> LAAMKNFAEQYAKRTDTYFCSDLSVTAVVIEGLARHKEELGSPLCPCRH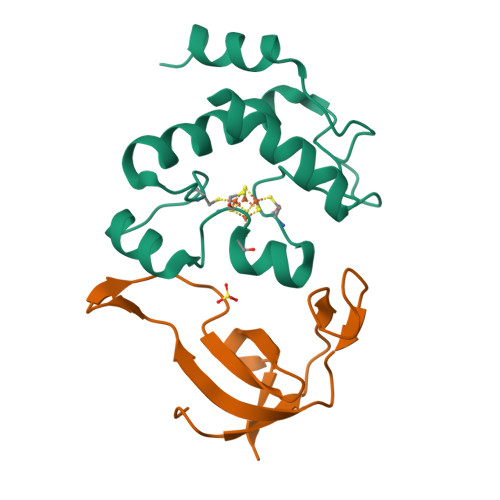YADKEAEVKNTFWNCPCVPMRERKECHCMLFLTPDNDFAGDAQGIPMETLEEKKASMA;> MNVGDRVRVTSSVVVYHHPEHAKTAFDLQGMEGEVAAVLTGWQGRPISANLPVLVKFEQRFKAHFRPDEVTLI(3R,5R,7R)-octane-1,3,5,7-tetracarboxylic 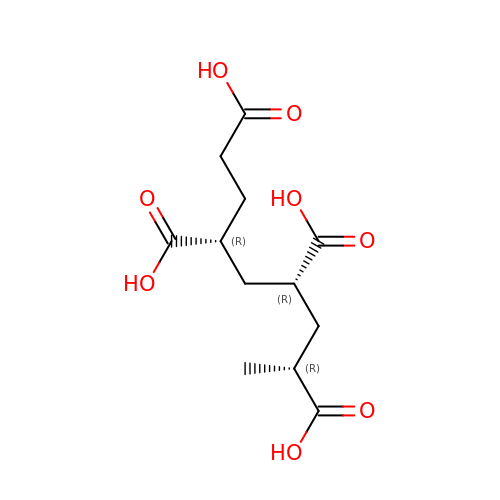acid | C12 H18 O8 | UEYGDIASMOPQFG-BWZBUEFSSA-N>[3x]MAILGLGTDIVEIARIEAVIARSGDRLARRVLSDNEWAIWKTHHQPVRFLAKRFAVKEAAAKAFGTGIRNGLAFNQFEVFNDELGKPRLRLWGEALKLAE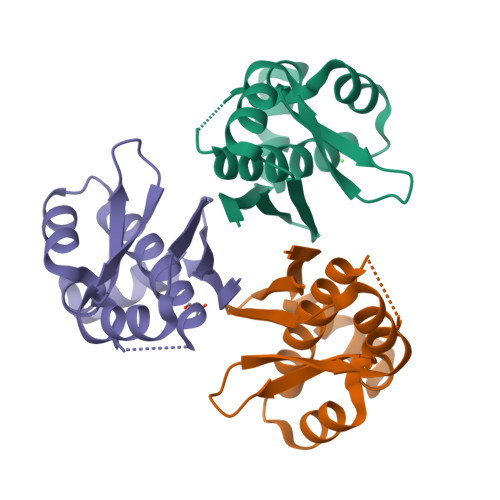KLGVANMHVTLADERHYACATVIIES>[4x]GPLGSDFPQHSQHVLEQLNQQRQLGLLCDCTFVVDGVHFKAHKAVL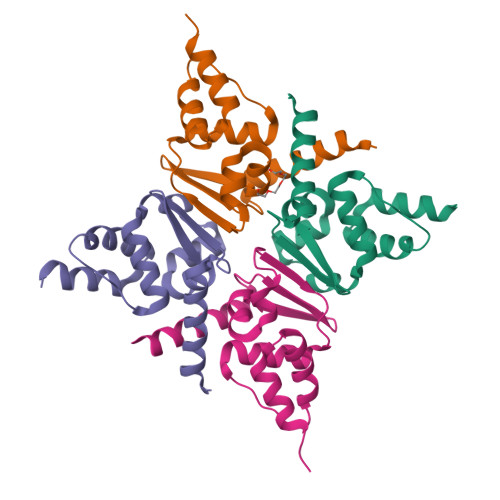AACSEYFKMLFVDQKDVVHLDISNAAGLGQVLEFMYTAKLSLSPENVDDVLAVATFLQMQDIITACHALKSLA Ribosomes are the protein synthesis machineries of the cell, which translate genetic codes on mRNA into protein in all living species. Here, we have used single particle cryo-EM reconstruction to determine the endogenous structures of M. smegmatis (Ms) 70S ribosome in the hibernating state, trans-translating state, and P-tRNA bound P/P state. Ms ribosome shares the conserved ribosomal architecture with Ec ribosome. With a conserved core structure of ribosome, mycobacterial ribosome exhibits various unique extensions in its rRNAs and r-proteins.

The 70S-log cryo-EM dataset resulted in one major class of 70S ribosome (with P-tRNA, 99.4% particles) resolved to 3.4 Å (the P/P state) and one minor class of trans-translating 70S ribosome with the presence of a tmRNA-SmpB (0.6% particles) resolved to 12.5 Å. Surprisingly, we were able to identify this minor population of about 0.6% of 70S ribosome in trans-translational state in the 70S-log dataset. We believe that use of a bigger dataset of about 391,000 particles with a careful 3D classification allowed us to identify this state. Because of the limited number of particles (~1,300), the trans-translating map could only be refined to an average resolution of 12.5 Å. Docking of the known tmRNA bound 70S models of Ec and Tth in our map enabled us to identify that our trans-translation state represents the resumed state with tRNA bound at A-site and tmRNA-SmpB complex at P-site. Ms tmRNA is 369 nt long and shares 50.7% sequence identity with Tth (349 nt) and 51.5% with Ec (363 nt). Secondary structure of Ms tmRNA is presented in the Supplementary Fig. S11. tmRNA is consisted of four pseudoknots (PK 1–4), two helices (H2 and H5), one tRNA like domain (TLD), and one mRNA like domain (MLD). The four pseudoknots of tmRNA form an arc-like structure reaching from the beak of SSU to the mRNA entry channel while the two helices (H2 and H5) help in the accurate positioning of tmRNA on to the ribosome. The TLD is formed by the 5′ and 3′ ends of tmRNA and together with the small protein B (SmpB) mimic the tRNA structure. SmpB is a conserved protein in prokaryotes and an essential component of trans-translation. This 18.2 kDa basic protein (pI: 10.27) stabilizes tmRNA binding at the A- and P-tRNA binding sites and compensates for the D-stem and the anticodon loop of tRNA in tmRNA and is an indispensable element in trans-translation.

> MTKKSASSNNKVVATNRKARHNYTILDTYEAGIVLMGTEVKSLREGQASLADAFATVDDGEIWLRNVHIAEYHHGTWTNHAPRRNRKLLLHRKQIDNLIGKIRDGNLTLVPLSIYFTDGKVKVELALARGKQAHDKRQDLARRDAQREVIRELGRRAKGKI>[2x]GAMGSDEQPHIGNYRLLKTLGKGNFAKVKRARHILTGREVAIKIIDKTQLNPTSLQKLFREVRIMK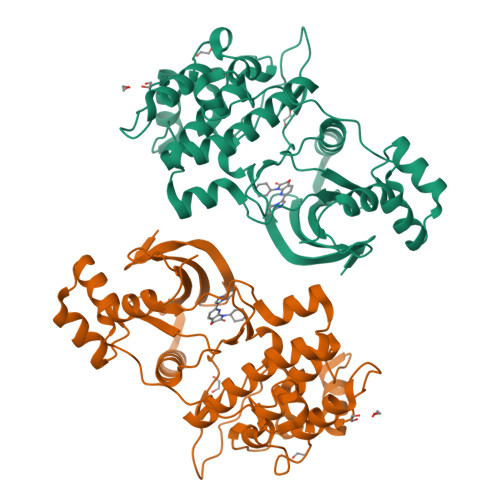ILNHPNIIKLFEVIETEKTLYLIMEYASKGEVYDYLVEHGRMKEKEARSKFRQIVSAVQYCHQKRIVHRDLKAENLLLDADMNIKIADFGFSNEFTKGGKLDTFCGSPPYAAPELFQGKKYDGPEVDVWSLGVILYTLVSGSLPFDGQNLKELRERVLRGKYRIPFYMSTDCENLLKRFLVLNPIKRGTLEQIMKDRWINAGHEEDELKPFVEPELDISDQKRIDIMVGMGYSQEEIQESLSKMKYDEITATYLLLGRKSSE>[2x]REWFLHRNSLI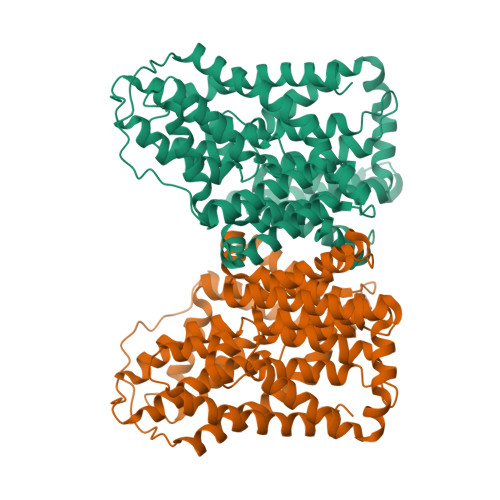VLADVALFLALYHFLPFEHNVVLGISMLAFIAVLWLTEALHVTVTAILVPVMAVFFGIFETQAALNNFANSIIFLFLGGFALAAAMHHQGLDKVIADKVLAMAQGKMSVAVFMLFGVTALLSMWISNTATAAMMLPLVLGVLSKVDADKQRSTYVFVLLGVAYSASIGGIATLVGSPPNAIAAAEVGLSFTDWMKFGLPTAMMMLPMAIAILYFLLKPTLNGMFELDRAPVNWDKGKVVTLGIFGLTVFLWIFSSPINAALGGFKSFDTLVALGAILMLSFARVVHWKEIQKTADWGVLLLFGGGLCLSNVLKQTGTSVFLANALSDMVSHMGIFVVILVVATFVVFLTEFASNTASAALLIPVFATVAEAFGMSPVLLSVLIAVAASCAFMLPVATPPNAIVFASGHIKQSEMMRVGLYLNIACIGLLTAIAMLFWQ>[9x]MDAEGLALLLPPVTLAALVDSWLREDCPGLNYAALVSGAGPSQAALWAKSPGVLAGQPFFDAIFTQLNCQV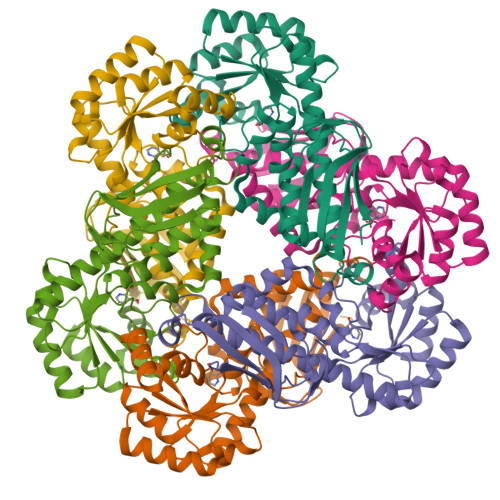SWFLPEGSKLVPVARVAEVRGPAHCLLLGERVALNTLARCSGIASAAAAAVEAARGAGWTGHVAGTRKTTPGFRLVEKYGLLVGGAASHRYDLGGLVMVKDNHVVAAGGVEKAVRAARQAADFALKVEVECSSLQEAVQAAEAGADLVLLDNFKPEELHPTATVLKAQFPSVAVEASGGITLDNLPQFCGPHIDVISMGMLTQAAPALDFSLKLFAKEVAPVPKIHLEHHHHHH1,3-oxazol-4-ylmethanamine | C4 H6 N2 O | 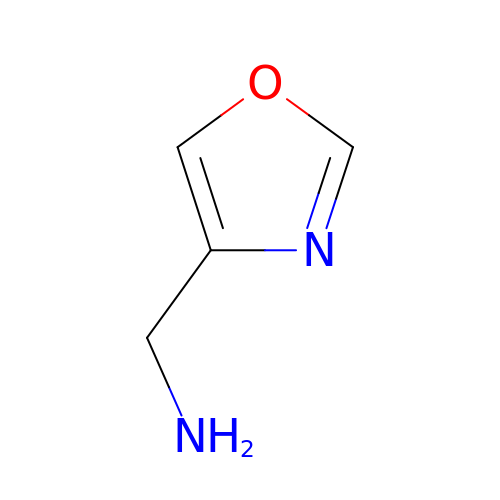ULZXEYFKBUPRQM-UHFFFAOYSA-N>[3x]MNVASRVVVNADRVKGTINRNIYGHFSEHLGRCIYEGLWVGEDSPIPNT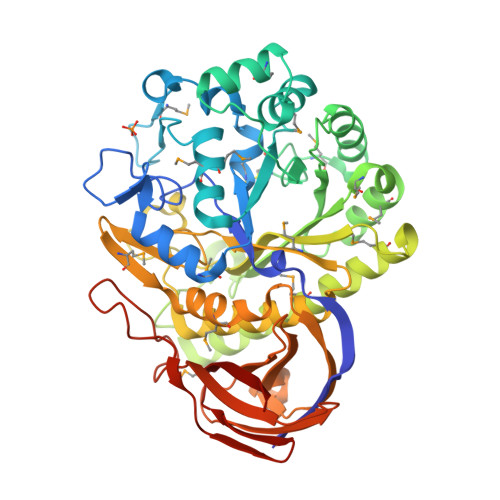NGIRNDVLEALKQMKIPVLRWPGGCFADEYHWKDGVGPREKRKRMVNTHWGGVIENNHFGTHEFMMLCELLGCEPYISGNVGSGTVQEMSEWVEYITFDGESPMANWRRENGREKPWRIKYWGVGNENWGCGGNMRAEYYADLYRQFQTYLRNYGDNKLHKIACGANTADYHWTEVLMKQAAPFMHGLSLHYYTVPGPWEKKGPATGFTTDEWWVTLKKALFMDRLVTKHSAIMDVYDPDKRIDLIVDEWGTWYDVEPGTNPGFLYQQNSIRDALVAGATLHIFHRHCDRVRMANIAQLVNVLQSVILTEGERMLLTPTYHVFNMFKVHQDAELLDTWESVERTGPEGELPKVSVSASRAADGKIHISLCNLDFETGASVDIELRGLNGGVSATGTTLTSGRIDGHNTFDEPERVKPAPFRDFKLEGGHLNASLPPMSVTVLELTAG>[2x]MGDKPIWEQIGSSFIQHYYQLFDNDRTQLGAIYIDASCLTWEGQQFQGKAAIVEKLSSLPFQKIQA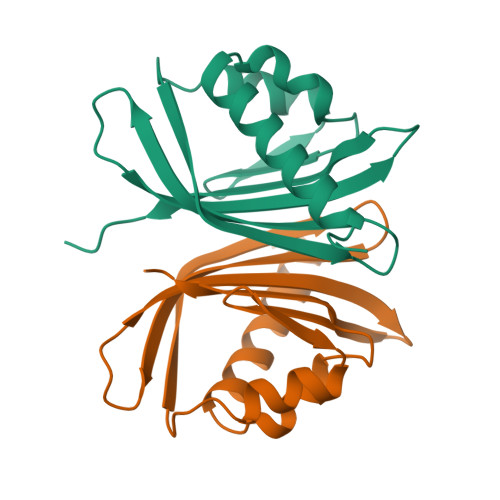SITAQDHQPTPDSCIISMVVGQLKADEDPIMGFHQMFLLKNINDAWVCTNDMFRLALHNFG> MTENILRKSDEEIQKEITARVK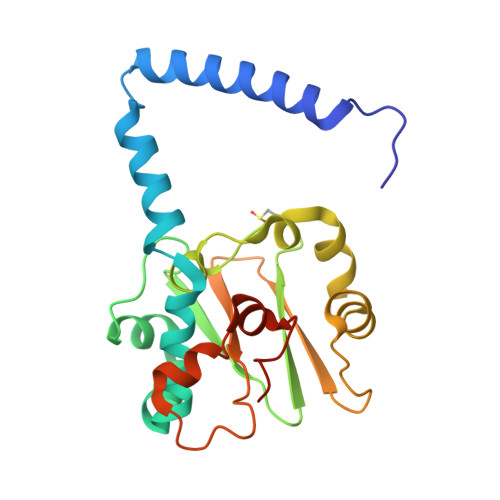ALESMLIEQGILTTSMIDRMAEIYENEVGPHLGAKVVVKAWTDPEFKKRLLADGTEACKELGIGGLQGEDMMWVENTDEVHHVVVCTLCSCYPWPVLGLPPNWFKEPQYRSRVVREPRQLLKEEFGFEVPPSKEIKVWDSSSEMRFVVLPQRPAGTDGWSEEELATLVTRESMIGVEPAKAVHHHHHH>[2x]INTITYDAGNTTINKYATFMESLRNEAKDPSLQCYGIPMLPNNSST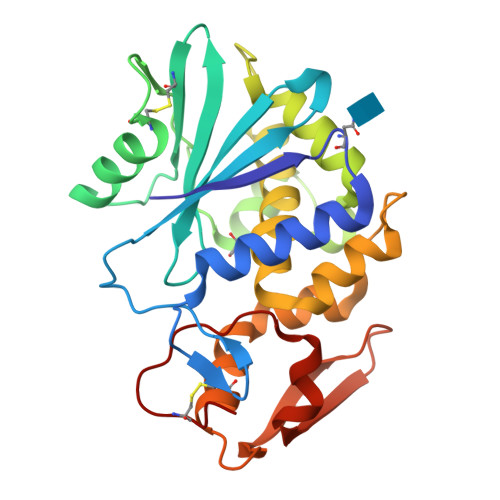IKYLLVKLQGASQKTITLMLRRNNLYVMGYSDPFNGNCRYHIFNDITGTERTNVENTLCSSSSSRDAKPINYNSLYSTLEKKAEVNSRSQVQLGIQILSSDIGKISGQSSFTDKTEAKFLLVAIQMVSEAARFKYIENQVKTNFNRDFSPNDKILDLEENWGKISTAIHDATNGALPKPLELKNADGTKWIVLRVDEIKPDMGLLNYVNGTCQTT>[4x]GAMCRKSRNCRNPPRSGDAQQ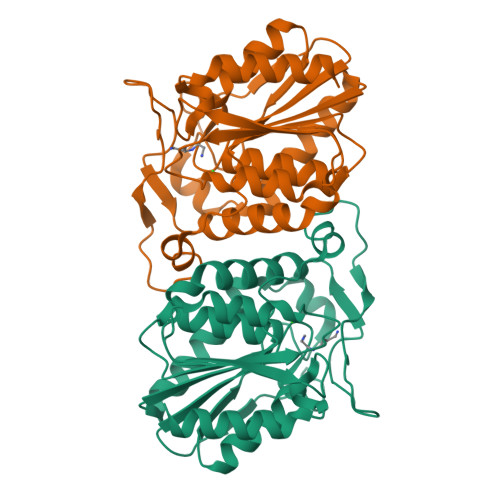RPRERSGSGMSTTPLQVLPGAEPLYSVGSRIGVLVSHGFTGSPQSMRFLAEGFARAGYTVATPRLTGHGTTPAEMAASTASDWTADIVAAMRWLEERCDVLFMTGLSMGGALTVWAAGQFPERFAGIMPINAALRMESPDLAALAFNPDAPAELPGIGSDIKAEGVKELAYPVTPVPAIKHLITIGAVAEMLLPRVKCPALIIQSREDHVVPPHNGELIYNGIGSTEKELLWLENSYHVATLDNDKELILERSLAFIRKH> TAKEACVAKFGPLPSKWQMEPPKPSCVNKISDWKLKILQNGLYIIYGQVA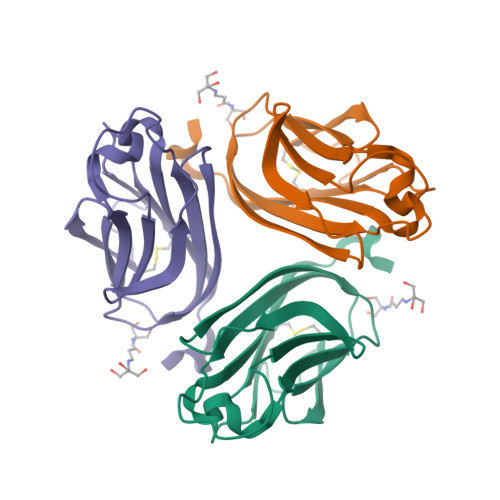PDPTYKGFAPFEVQLCKNKEAIQTLTNNSKIQNLGGIYEFDAGDIIELRFNSDDQVLKNNTYWGIVLLVTPQFSS>[2x]GNIESIENLQGIRALQQQAPQLLSSGLPNEQQFSLLKQAGVDVVINLMPDSSKDAHPDEGKLVTQAGMDYVYIPVDWQNPKVEDVEAFFAAMDQHKGKDVLVHCLANYRASAFA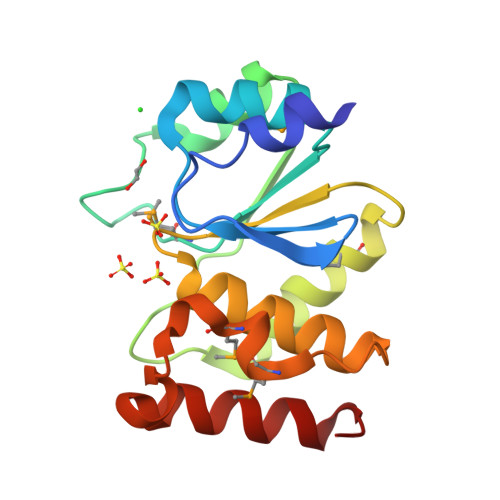YLYQLKQGQNPNMAQTMTPWNDELAIYPKWQALLTEVSAKYGH> GSHMQGQSPIKDQEMKELIRRSQEGDQEARDEIIEKNMRLVWSVVQRFLNRGYEADDLFQIGCIGLLKSVDKFDLSYDVKFSTYAVPMIIGEIQRFLRDDGTVKVSRSLKEMGNKIRKAKDELSKTRGRAPTVTEIADHLG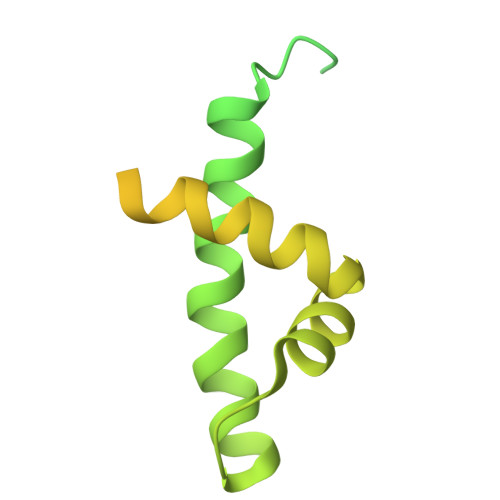ISPEDVVLAQEAVRLPTSIHETVYENDGDPITLLDQIADADEASWFDKIALKKAIEELDERERLIVYLRYYKDQTQSEVASRLGISQVQMSRLEKKILQHIK>GSHMPIERIVQVDLDYIYDPDPEQQNRNLGQLIDRMKDLAPSAVYLQAFADPKGDGDITEVYFPNRHLPMRADLFNRVAWQLKTRAGVMVYAWLPVLTFSVPPGNPAYGKVVQSTTRKPGERGLGSPTRLSPFHPDAHRVISEIYEDLAKAAHFDGLLFHDDAVLDDTEDSSPEALATYQGWGLPPDIAAIRADPKLAQQWSKGKIRYLIDFTMHLRHIVSGYQNDR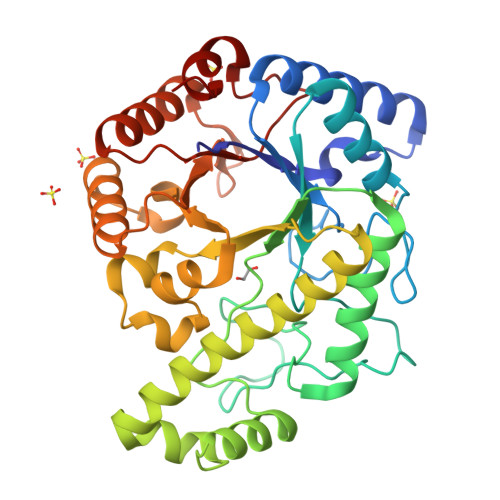DMVVARNLYAQPVLDPVSEAWYGQSLPEFLKSYDFVALMAMPNMEGAARPEQWMRQLVAAVARQKGLDRTIFELQARDWRVGKPIDTEILRRQMVQLRSLGAINYGYYPDDFIANHPDAEALRDVMSLKS[2x]> DCPSGWSSYDGHCYQVFSDLKNWDDAESFCSGQHEGSRLASIHSREEEAFVGKMASRTLKYTSMWLGLNNPWKECKWEWSDDTRLDYKVWTRRPYCTVMVVKTDRIFWFNRGCEKSVSFVCK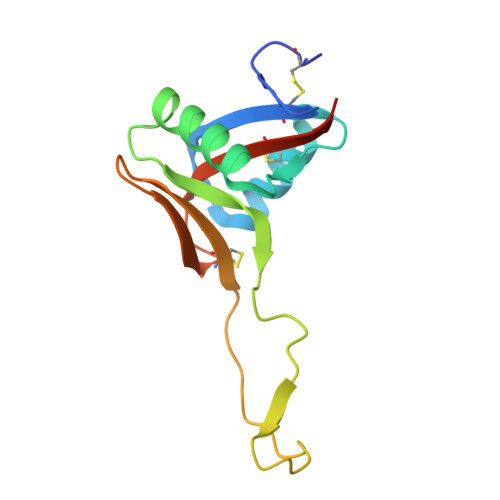FKAYSEDAAE> KQKPRYEIRWRVIESISPDGHEYIYVDPMQLPYDSRWEFPRDGLVLGRVLGSGAFGKVVEGTAYGLSRSQPVMKVAVKMLKPTARSSEKQALMSELKIMTHLGPHLNIVNLLGACTKSGPIYIITEYCFYGDLVNYLHKNRDSFLSHKKKSMLDSEVKNLLSDDNSEGLTLLDLLSFTYQVARGMEFLASKNCVHRDLAARNVLLAQGKIVKICDFGLARDIMHDSNYVSKGSTFLPVKWMAPESIFDNLYTTLSDVWSYGILLWEIFSLGGTPYPGMMVDSTFYNKIKSGYRMAKPDHATSEVYEIMVKCWNSEPEKRPSFYHLSEIVENLLPGQYKKSYEKIHLDFLKSD

Avapritinib is the only potent and selective inhibitor approved for the treatment of D842V-mutant gastrointestinal stromal tumors (GIST), the most common primary mutation of the platelet-derived growth factor receptor α (PDGFRA). Against this background, we solve the crystal structures of avapritinib in complex with wild-type and mutant PDGFRA and stem cell factor receptor (KIT), which provide evidence and understanding of inhibitor binding and lead to the identification of a sub-pocket (Gα-pocket). Furthermore, we report the identification of a sub-pocket (Gα-pocket) located in the N-lobe of the kinase domain, which is surrounded by amino acids of key regulatory elements such as the Gly-rich loop and the αC-helix.

In total, we obtained protein crystals suitable for structure determination which resulted in a total of 12 crystal structures: two apo-crystal structures and ten complex structures of KIT-wt, -T670I, and PDGFRA-T674I bound to avapritinib and to different ligands synthesized in our laboratory. Similar results were also obtained for apo-PDGFRA-wt and -T674I, showing that the water molecule is located near the gatekeeper in the case of the PDGFRA-wt structure but not in the PDGFRA-T674I structure.> MIQKGLEGVKICESSICYLDGI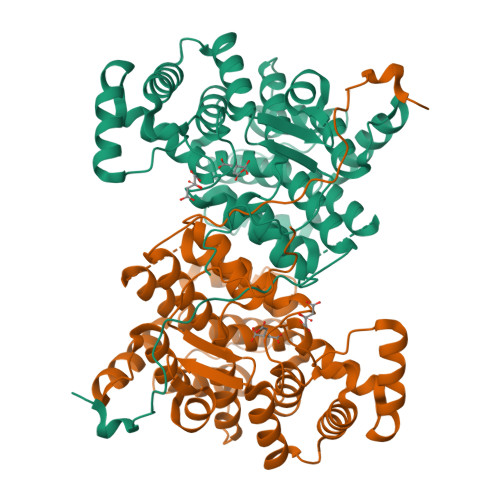NGRLYYRGIPVEELAEKSTFEETAYFLWYGKLPTKSELEEFKRKMADYRELPAEALGILYHLPKNLHYIDVLKIFLSIHGSMDGNDEDLREKAIRVASVFPTILAYYYRYSKGKELIRPRKDLSHVENFYYMMFGERNEKIRLLESAFILLMEQDINASTFAALVIASTLSDLYSCIVGALGALKGPLHGGASEKVPPMLEEIGSEDRVEEFVQKCLKEKRKIMGFGHRVYKTYDPRAVFLKRVLQEHFPDSKLFRIASKLEEYIVSNKIKNIYPNVDLYSSVLFEELGFPRNMFTALFATARVVGWTAHVIEYVSDNKLIRPTSEYVGPMDVEYIPIERRDENG> AFVVTDNC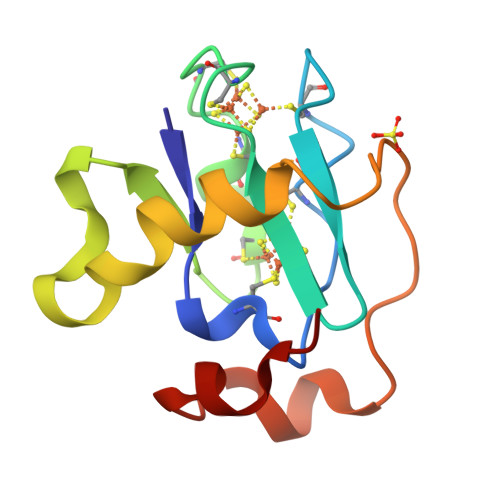IKCKYTDCVEVCPVDCHYEGPNFLVIHPDECIDCALCEPECPAQAIFSEDEVPEDMQEFIQLNAELAEVWPNITEKKDPLPDAEDWDGVKGKLQHLER>MASMTGGQQMGRGSMSRDPLPFFPPLYLGGPEITTENCEREPIHIPGSIQPHGALLTADGHSGEVLQMSLNAATFLGQEPTVLRGQTLAALLPEQWPALQAALPPGCPDALQYRATLDWPAAGHLSLTVHRVGELLILEFEPTEAWDSTGPHALRNAMFALESAPNLRALAEVATQTVRELTGFDRVMLYKFAPDATGEVIAEARREGLHAFLGHRFPASDIPAQARALYTRHLLRLTADTRAAAVPLDPVLNPQTNAPTPLGGAVLRATSPMHMQFLRNMGVGSSLSVSVVVGGQLWGLIACHHQTPYVLPPDLRTTLEYLGRLLSLQVQVKEAADVAAFRQSLREHHARVALAAAHSLSPHDTLSDPALDLLGLMRAGGLILRFEGRWQTLGEVPPAPAVDALLAWLETQPGALVQTDALGQLWPAGADLAPSAAGLLAISVGEGWSECLVWLRPELRLEVAWGGATPDQAKDDLGPRHSFDTYLEEKRGY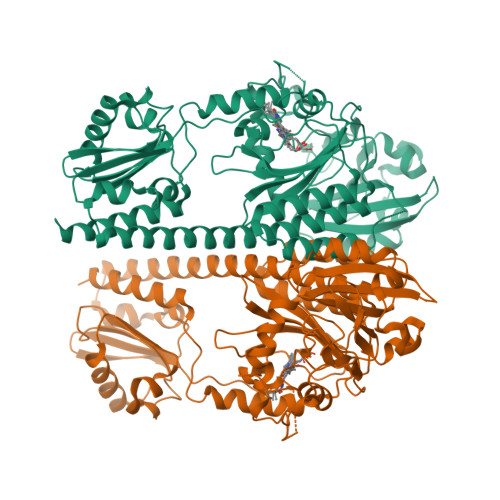AEPWHPGEIEEAQDLRDTLTGALEHHHHHH[4x]>SPGQDIQLIPPLINLLMSIEPDVIYAGHDNTKPDTSSSLLTSLNQLGERQLLSVVKWSKSLPGFRNLHIDDQITLIQYSWMSLMVFGLGWRSYKHVSGQMLYFAPDLILNEQRMKESSFYSLCLTMWQIPQEFVKLQVSQ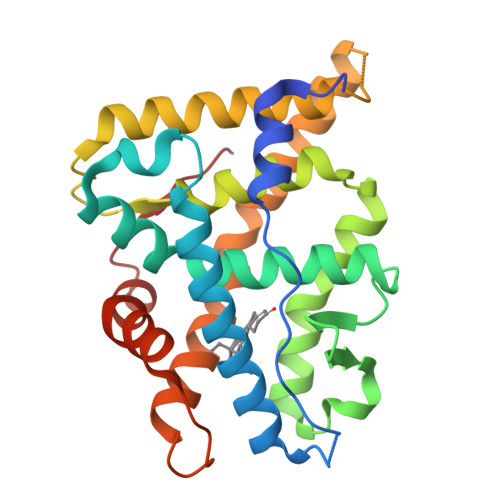EEFLCMKVLLLLNTIPLEGLRSQTQFEEMRSSYIRELIKAIGLRQKGVVSSSQRFYQLTKLLDNLHDLVKQLHLYCLNTFIQSRALSVEFPEMMSEVIAAQLPKILAGMVKPLLFHKK[2x]>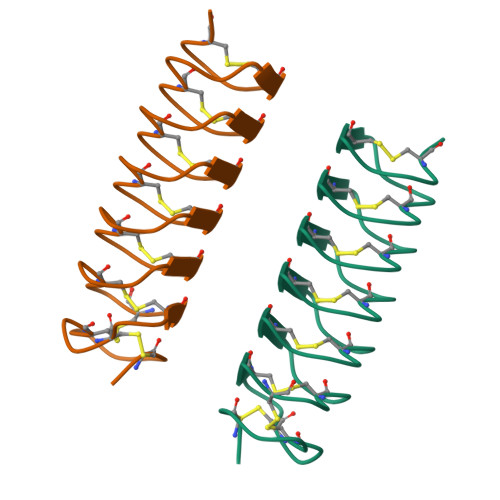QCTGGADCTSCTGACTGCGNCPNAVTCTNSQHCVKANTCTGSTDCNTAQTCTNSKDCFEANTCTDSTNCYKATACTNSSGCPGH[2x]> GSSHSSANEDMPVERILEAELAVEPKTETYVEANMGLNPSSPNDPVTNICQAADKQLFTLVEWAKRIPHFSELPLDDQVILLRAGWNELLIASFSHRSIAVKDGILLATGLHVHRNSAHSAGVGAIFDRVLTELVSKMRDMQMDKTELGCLRAIVLFNPDSKGLSNPAEVEALREKVYASLEAYCKHKYPEQPGRFAKLLLRLPALRSIGLKCL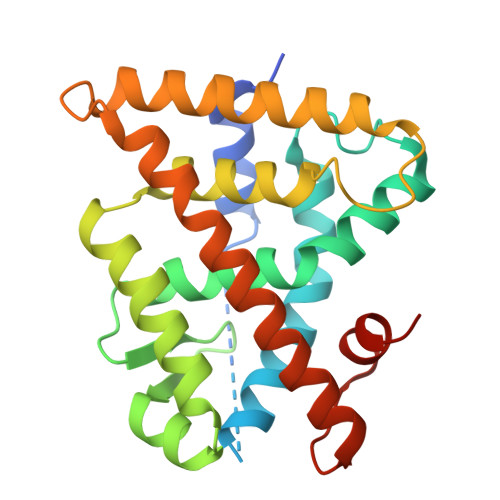EHLFFFKLIGDTPIDTFLMEMLEAPHQMT>[2x]MEDPLIGRDSLGGGGTDRVRRSEAITHGTPFQKAAALVDLAEDGIGLPVEILDQSSFGESARYYFIFTRLDLIWSLNYFALLFLNFFEQPLWCEKNPKPSCKDRDYYYLGELPYLTNAESIIYEVITLAILLVHTFFPISYEGSRIFWTSRLNLVKVACVVILFVDVLVDFLYLSPLAFDFLPFRIAPYVRVIIFILSIRELRDTLVLLSGMLGTYLNILALWMLFLLFASWIAFVMFEDTQQGLTVFTSYGATLYQMFILFTTSNNPDVWIPAYKSSRWSSVFFVLYVLIGVYFVTNLILAVVYDSFKEQLAKQVSGMDQMKRRMLEKAFGLIDSDKNGEIDKNQCIKLFEQLTNYRTLPKISKEEFGLIFDELDDTRDFKINKDEFA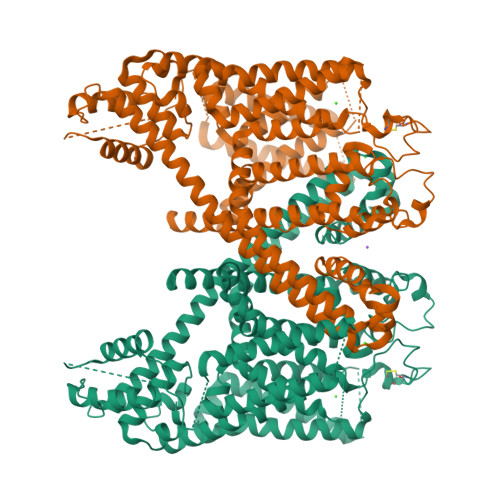DLCQAIALRFQKEEVPSLFEHFPQIYHSALSQQLRAFVRSPNFGYAISFILIINFIAVVVETTLNIEESSAQKNWQVAEFVFGWIYVLEMALKIYTYGFENYWREGANRFDFLVTWVIVIGETATFITPDENTFFSNGEWIRYLLLARMLRLIRLLMNVQRYRAFIATFITLIPSLMPYLGTIFCVLCIYCSIGVQVFGGLVNAGNKKLFETELAEDDYLLFNFNDYPNGMVTLFNLLVMGNWQVWMESYKDLTGTWWSITYFVSFYVITILLLLNLVVAFVLEAFFTELDLEEEEKCQGQDSQEKRNRRRSAGSKSRSQRVDTLLHHMLGDELSKPECSTSDT> MSHQERLQSKSLHLSPQEQSASYQDRRQSWRRASMKETNRRKSLHPIHQGITELSRSISVDLAESKRLGCLLLSSFQFSIQKLEPFLRDTKGFSLESFRAKASSLSEELKHFAD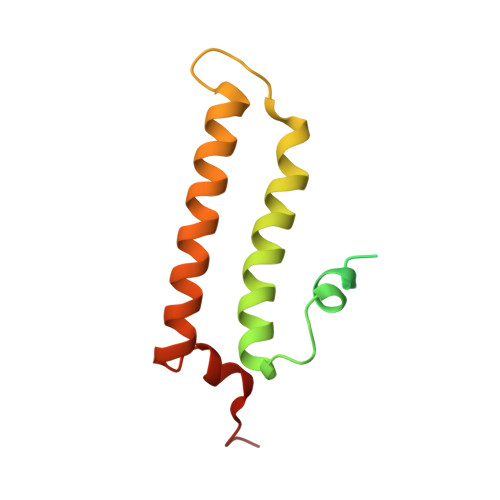GLETDGTLQKCFEDSNGKAS> MHHHHHHAMGKQVSSRGGKSKKLSVTPPSSNGINEELSEVLQTLQDEFGQMSFDHQQLAKLIQESPTVELKDKLECELEALVGRMEAKANQITKVRKYQAQLEKQKLEKQ

Located in the inner layer of PCM, Cep57 is a conserved protein in vertebrates that features coiled-coil domains at the N and C termini. Cep57 maintains centriole engagement for accurate centrosome biogenesis. Our work elucidates how human PCM protein Cep57 assembles into micron-sized biomolecular condensates through liquid–liquid phase separation by employing various tools in vitro. Both purified Cep57 and Cep57S undergo LLPS, driven by at least three interacting regions, including NTD, LMN motif, and CTD. Here, we demonstrate that a crucial centrosomal protein, Cep57, self-assembles through multivalent interactions.

To obtain atomic structure information on Cep57, we determined a crystal structure of the Cep57C at 2.10 Å resolution in the space group of P6422. The Cep57C adopts a helix–turn–helix fold, with one protomer in the asymmetric unit, forming a symmetric dimer. The ordered residues span from 354 to 428, with Helix 1 comprising residues 356 to 387, and Helix 2 comprising residues 391 to 427. The dimer interface is composed of two universally conserved F371 and F376 in Helix 1, whose benzyl rings pack well in a near 90-degree orientation with the centroid distance of 5.6 Å, a very stable π–π stacking interaction. Cep57C is also a dimer in 150 mM salt based on the analysis of SEC-MALS (size exclusion chromatography coupled with multiangle light scattering). To test whether dimerization is important for LLPS, we performed structure–function analyses by replacing F371 and F376 with Ala in Cep57C and Cep57S, referred to as Cep57C-FF and Cep57S-FF. SEC-MALS data showed that the size of Cep57C-FF mutant decreased to ~17 kDa, indicating it is a mixed population of dimer and monomer. Furthermore, the FF mutation reduced the thermal stability of Cep57C by 11.5 degrees, while the secondary structure remains similar to the wild-type Cep57C as monitored by circular dichroism. Compared with the wild-type Cep57S, the FF mutation decreased the condensate size, partition coefficient, and critical concentration for LLPS. Therefore, Cep57C dimerization is essential to promote Cep57 condensation.> GSSHHHHHHSSGLVPRGSMSTSWSDRLQNAADMPANMDKHALKKYRREAYHRVFVNRSLAMEKIKCFGFNMDYTLAVYKSPEYESLGFELTVERLVSIGYPQELLSFAYDSTFPTRGLVFDTLYGNLLKVDAYGNLLVCAHGFNFIRGPETREQYPNKFIQRDDTERFYILNTLFNLPETYLLACLVDFFTNCPRYTSCETGFKDGDLFMSYRSMFQDVRDAVDWVHYKGSLKEKTVENLEKYVVKDGKLPLLLSRMKEVGKVFLATNSDYKYTDKIMTYLFDFPHGPKPGSSHRPWQSYFDLILVDARKPLFFGEGTVLRQVDTKTGKLKIGTYTGPLQHGIVYSGGSSDTICDLLGAKGKDILYIGDHIFGDILKSKKRQGWRTFLVIPELAQELHVWTDKSSLFEELQSLDIFLAELYKHLDSSSNERPDISSIQRRIKKVTHDMDMCYGMMGSLFRSGSRQTLFASQVMRYADLYAASFINLLYYPFSYLFRAAHVLMPHESTVEHTHVDINEMESPLA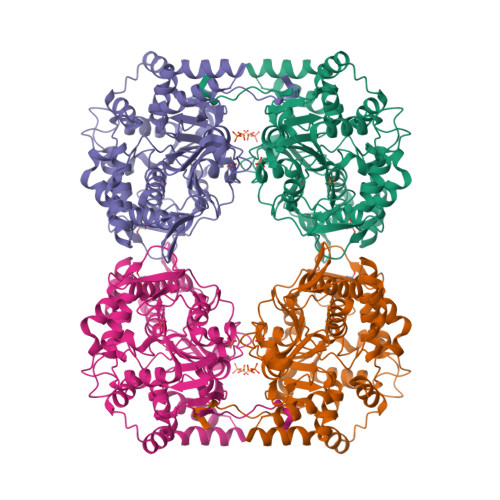TRNRTSVDFKDTDYKRHQ> MGLTIGVDIGGTKIAAGVVDEEGRILSTFKVATPPTAEGIVDAICAAVAGASEGHDVEAVGIGAAGYVDDKRATVLFAPNIDWRHEPLKDKVEQRVGLPVVVENDANAAAWGEYRFGAGQGHDDVIC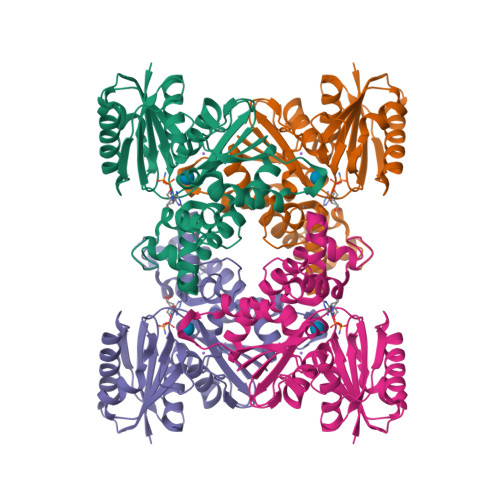ITLGTGLGGGIIIGNKLRRGRFGVAAEFGHIRVVPDGLLCGCGSQGCWEQYASGRALVRYAKQRANATPENAAVLLGLGDGSVDGIEGKHISEAARQGDPVAVDSFRELARWAGAGLADLASLFDPSAFIVGGGVSDEGELVLDPIRKSFRRWLIGGEWRPHAQVLAAQLGGKAGLVGAADLARQGLEHHHHHH>[3x]MSKINDYYSDPKEYIESKYYDALFSIHTPLAYFVKSNLVRLKNTCRTKYGSDSYKIAYQAMLQKFLLSIVQFKDRHDNRLLLEPF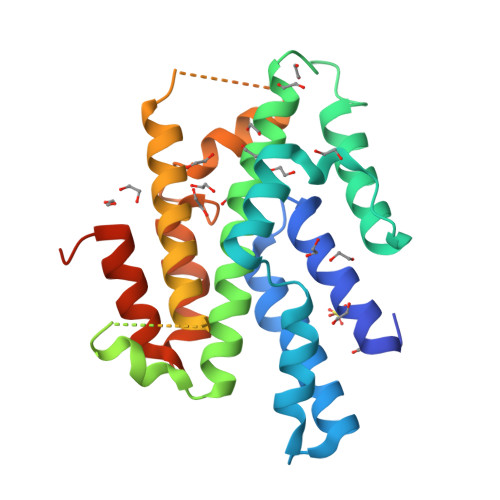SSPIADEKRKNCLTKFVIQDENKNSSTIADLCVVLKSREIKLQILLLLEIIGLNDLDWNFRDFEKKYKLKLKKRSLNLTKKGLVRRRSKKKTSEKDKGIERITTSLDYCEQLDLYLDRACILDILLSSETPNPDAIEASNGTIQEHKKNILDKSKEASLVGFINYVLIPYFNKKVPHAVEFIIQKLKGPSMRPKRALKKLEHHHHHH> MTTVGFDVAARLGTLLTAMVTPFSGDGSLDTATAARLANHLVDQGCDGLVVSGTTGESPTTTDGEKIELLRAVLEAVGDRARVIAGAGTYDTAHSIRLAKACAAEGAHGLLVVTPYYSKPPQRGLQAHFTAVADATELPMLLYDIPGRSAVPIEPDTIRALASHPNIVGVKDAKADLHSGAQIMADTGLAYYSGDDALNLPWLAMGATGFISVIAHLAAGQLRELLSAFGSGDIATARKINIAVAPLCNAMSRLGGVTLSKAGLRLQGIDVGDPRLPQVAATPEQIDALAADMRAASVLR

Next, L-β-aspartyl-4-phosphate is reduced to L-aspartate-beta-semialdehyde (ASA) catalyzed by aspartate semialdehyde dehydrogenase. This is followed by a Schiff base formation with pyruvate and addition of ASA to form (4S)-4-hydroxy-2,3,4,5-tetrahydro-(2S)-dipicolinate (HTPA) catalyzed by dihydrodipicolinate synthase (Mtb-DapA)8. Mtb-DapA belongs to the subfamily of N-acetylneuraminate lyase (α/β)8 proteins. It contains an N-terminal (α/β)8 TIM barrel catalytic core and an α-helical C-terminal domain19. The active site residues Thr54, Thr55, Tyr143, Arg148 and Lys171 of Mtb-DapA are largely conserved among its homologues.

The structure of Mtb-rDapA in complex with α-KPA was solved at 2.4 Å resolution. The Mtb-rDapA-α-KPA complex structure comprises a monomer of the polypeptide in P42212 space group. Hence, the residue Tyr117 that completes the catalytic triad could not be located closer to the active site. The structure reveals the presence of α-KPA at hydrogen bonding distance from the residues Thr54, Tyr143 and Lys171. In addition, α-KPA also forms hydrogen bonding interactions with Thr55, Arg148 and Gly194. Alpha-KPA occupies the position of the substrate pyruvate and thus could prevent the formation of a Schiff base with pyruvate, which is the first step of the ping-pong reaction. The Mtb-DapA and Mtb-rDapA-α-KPA complexed structures superpose very well with an RMSD of 0.3 Å, indicating an apparent lack of conformational changes in the protein upon ligand binding. The proportion of inhibition measured at different concentrations of the analogues showed that the IC50 for α-KPA was 21 μM and the inhibition constant Ki was 32.5 μM at 500 μM pyruvate and 400 μM ASA. The IC50 of Mtb-rDapA pre-incubated with pyruvate was 160 μM, which is nearly 8 fold higher compared to pre-incubation with α-KPA. These results suggest that α-KPA competes with pyruvate for a binding site in Mtb-rDapA. Our results show that α-KPA disrupts the oligomerization of Mtb-rDapA thereby causing loss of enzyme activity.>MEQTEKSKVYAENGLLEKIKLCLSKKPLPSPTERKKFDHDFAISTSFHGIHNIVQNRSKIRRVLWLVVVLGSVSLVTWQIYIRLLNYFTWPTTTSIEVQYVEKMEFPAVTFCNLNRFQTDAVAKFGVIFFLWHIVSKVLHLQEITANSTGSREATDFAASHQNFSIVEFIRNKGFYLNNSTLLDCEFFGKPCSPKDFAHVFTEYGNCFTFNHGETLQAKRKVSVSGRGLSLLFNVNQEAFTDNPALGFVDAGIIFVIHSPKKVPQFDGLGLLSPVGMHARVTIRQVKTVHQEYPWGECNPNIKLQNFSSYSTSGCLKECKAQHIKKQCGCVPFLLPGYGIECDLQKYFSCVSPVLDHIEFKDLCTVGTHNSSCPVSCEEIEYPATISYSSFPSQKALKYLSKKLNQSRKYIRENLVKIEINYSDLNYKITQQQKAVSVSELLADLGGQLGLFCGASLITIIEIIEYLFTNFYWICIFFLLKISEMTQWTPPPQNHLGNKNRIEEC[3x]

The bile acid-sensitive ion channel (BASIC) is the least understood member of the mammalian epithelial Na+ channel/degenerin (ENaC/DEG) superfamily of ion channels, which are involved in a variety of physiological processes. There is, however, a conserved architecture among other members of the ENaC/DEG superfamily. These trimeric channels resemble a chalice in which a large extracellular domain (ECD) connects to a slender transmembrane domain (TMD) via linkers at the membrane interface. In this study, we used single-particle cryo-EM to determine the structure of hBASIC in the membrane-like environment of lipid nanodiscs, confirming its global adherence to the canonical ASIC fold. By determining structures in the presence and absence of Ca2+, we identified a single Ca2+-bound, non-conducting conformation of hBASIC, as well as both conducting and non-conducting conformations of Ca2+-free BASIC, revealing unexpected Ca2+-dependent conformational changes.

To investigate the structure of hBASIC in its resting state, we performed single-particle cryo-EM analysis of hBASIC reconstituted in nanodiscs in the presence of 2 mM Ca2+o, revealing a single conformation with a global resolution of 2.89 Å. The resulting density map enabled residues 29-479 of hBASIC to be fitted, with unambiguous assignment of most side chains. Five N-linked glycan molecules per protomer were assigned at sites predicted from sequence analysis and deglycosylation assays confirmed heavy glycosylation of hBASIC. The overall architecture of hBASIC in the presence of Ca2+ adheres to the canonical ASIC fold, a conserved architecture among the ENaC/DEG superfamily of trimeric ion channels. In the Ca2+-closed structure, E440 and D444 are orientated upwards, forming two triangular antiprisms of negative electrostatic potential. In both the Ca2+-closed and EGTA-closed structures, this ‘glycine gate’ is impermeable to ions, with pore radii less than 1 Å and ~1.2 Å, respectively. The HG motif of the re-entrant loop points directly into the pore in the Ca2+-closed structure, obstructing the pathway of ions. Analysis of the Ca2+-closed hBASIC map revealed a cylindrical Ca2+ ion-like density at the apex of the channel pore, a feature that was absent in both EGTA maps. Docking a Ca2+ ion into the ion-like density in the Ca2+-closed BASIC map revealed ~4.0 Å distances between the carboxyl oxygens of residue E440 and the putative ion. Ca2+ inhibits channel activity by directly binding to the carboxyl ring at the top of the pore, stabilizing the closed conformation of the TMD, which in turn locks the β1-β2 linker in a conformation that sterically prevents reorientation of the β11-β12 linkers that underlie channel activation.>[2x]MGSSHHHHHHSSGLMDSLLGCGVSAAAREPVPRYLTSQPRVSEVAMQSAPLEQPAKRPRCDGSPRTPPSTPPATANLSADDDFQNTDLRTWEPEDVCSFLENRGFREKKVLDIFRDNKIAGSFLPFLDEDRLEDLGVSSLEERKKMIECIQQLSQSRIDLM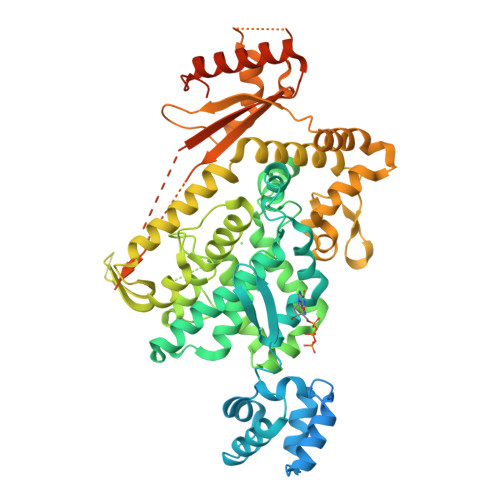KVFNDPIHGHIEFHPLLIRIIDTPQFQRLRYIKQLGGGYYVFPGASHNRFEHSLGVGYLAGCLVRALAEKQPELQISERDILCVQIAGLCHDLGHGPFSHMFDGRFIPRARPEKKWKHEQGSIEMFEHLVNSNELKLVMKNYGLVPEEDITFIKEQIMGPPITPVKDSLWPYKGRPATKSFLYEIVSNKRNGIDVDKWDYFARDCHHLGIQNNFDYKRFIKFARICEVEYKVKEDKTYIRKVKHICSREKEVGNLYDMFHTRNCLHRRAYQHKISNLIDIMITDAFLKADPYVEITGTAGKKFRISTAIDDMEAFTKLTDNIFLEVLHSTDPQLSEAQSILRNIECRNLYKYLGETQPKREKIRKEEYERLPQEVAKAKPEKAPDVELKAEDFIVDVINVDYGMEDKNPIDRVHFYCKSNSKQAVRINKEQVSQLLPEKFAEQLIRVYCKKKDGKSLDAAGKHFVQWCALRDFTKPQDGDIIAPLITPLKWNNKTSSCLQEVSKVKTCLKF>[2x]GSQSRIFYLRNFNNWMKSVLI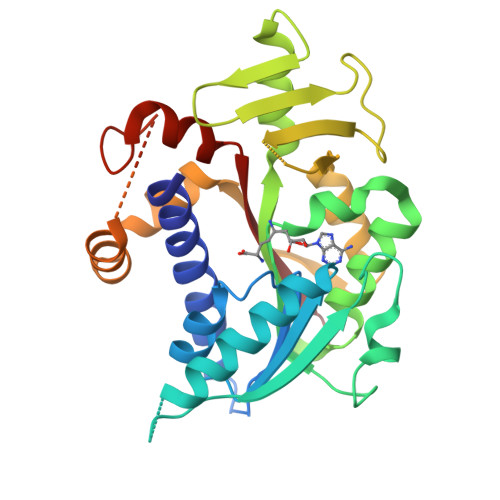GEFLEKVRQKKKRDITVLDLGCGKGGDLLKWKKGRINKLVCTDIADVSVKQCQQRYEDMKNRRDSEYIFSAEFITADSSKELLIDKFRDPQMCFDICSCQFVCHYSFESYEQADMMLRNACERLSPGGYFIGTTPNSFELIRRLEASETESFGNEIYTVKFQKKGDYPLFGCKYDFNLEGVVDVPEFLVYFPLLNEMAKKYNMKLVYKKTFLEFYEEKIKNNENKMLLKRMQALEPYPANESSKLVSEKVDDYEHAAKYMKNSQVRLPLGTLSKSEWEATSIYLVFAFEKQQ> MAQIWLWIGVIGMALGSIFFGIGAHNAKNERWKILFTINFFICAIATGLYLSMALGQGRSVIAGRPTVWVRYITWFLSTPLLILDLTFLGKTSLPITASLLGANAYMIATGFVATISADRTIGHIWYVVSCFAFLATVYLLVNQYRKQAERNYPQAKKVFRKLLSVHLVLWTLYPIVWLLGNTGFNAVNQGTETMFYTILDITSKVGFGFLSLNSMHTLEKNTESVSSYESSTI

Microbial rhodopsins (MRs) constitute a large family of photoactive 7 transmembrane (TM) α-helix proteins containing a retinal cofactor that is covalently bound to a conserved lysine residue in the 7th TM helix via a retinal Schiff base (RSB). The only characterized MR proposed to pump sulfate in addition to halides belongs to the cyanobacterium Synechocystis sp. PCC 7509 and is named Synechocystis halorhodopsin (SyHR). Here we present the crystal structure of SyHR in the ground state, the structure of its sulfate-bound form as well as two photoreaction intermediates, the K and O states.

Using red crystals of SyHR we solved the Cl−-bound structure of the protein at 1.57 Å resolution. The high-resolution structure reveals 126 protein-associated water molecules, including 27 inside SyHR, and 20 lipid fragments surrounding each protomer. The SyHR protomer consists of 7 transmembrane α-helices (A-G) connected by three intracellular and three extracellular loops like in other type I rhodopsins. A retinal chromophore is covalently bound to K205 and is in the all-trans configuration in the ground state of SyHR. As in archaeal HRs, a Cl− ion is found in the RSB region of SyHR in its ground state. The ion is coordinated by the T74 and S78 side chains of the characteristic TSD motif and also a water molecule (w401). The distance between the RSB nitrogen and the Cl− ion is 3.8 Å. Notably, the coordination of the chloride ion and water molecule w401 in SyHR is tighter compared to NpHR. The structure of SyHR in the ground state reveals two internal cavities at the cytoplasmic half of the protein, which we denoted as intracellular cavity 1 (IC1) and intracellular cavity 2 (IC2). The extracellular (EC) half of the SyHR protomer forms a large aqueous concave basin, protruding from the bulk to R71 (counterpart of R82 residue in BR) and, surprisingly, even further to the RSB counterion D201.>GNFEEPKATLTGKAIYDGEAVGVRSGSSEFALFQDGYALKGSIPVYIAQDGSYSVSLFNGDYKLVRMGNAPWERPSNDTIYITVRGNTVQDIPVTPYFFVRNVSFAKNGNKITARFTINKVVANANMENVGIYLGTGILTDEKQKEAELKLGNTVSLDQENTAEIEIPSGLVNESYLYARVGVKSDKSSEYCYSQS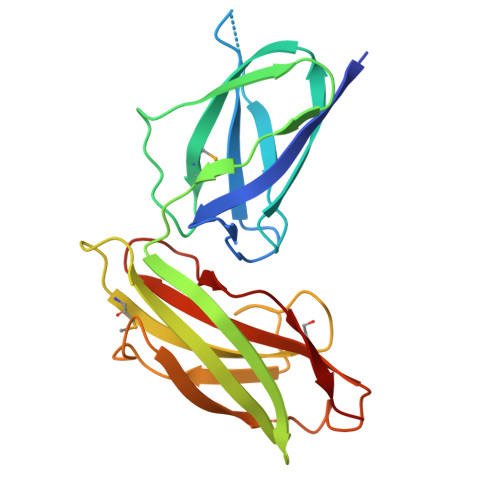IKVALK[14x]>[2x]MAGQLLFANFNQDNTSLAVGSKSGYKFFSLSSVDKLEQIYECTDTEDVCIVERLFSSSLVAIVSLKAPRKLKVCHFKKGTEICNYSYSNTILAVKLNRQRLIVCLEESLYIHNIRDMKVLHTIRETPPNPAGLCALSINNDNCYLAYPGSATIGEVQVFDTINLRAANMIPAHDSPLAALAFDASGTKLATASEKGTVIRVFSIPEGQKLFEFRRGVKRCVSICSLAFSMDGMFLSASSNTETVHIFKLETVGSGSFNQGRAFATVRLPFCGHKNICSLATIQKIPRLLVGAADGYLYMYNLDPQEGGECALMKQHRLDGSLET;>[2x]YAENEKDSRRRQARLQKELAEAAKE

The ATG12–5–16L1 complex is responsible for conjugating members of the ubiquitin-like ATG8 protein family to phosphatidylethanolamine in the growing autophagosomal membrane, known as the phagophore. ATG12–5–16L1 is recruited to the phagophore by a subset of the phosphatidylinositol 3-phosphate-binding seven-bladedß -propeller WIPI proteins. The two critical steps in autophagy initiation, PI 3-phosphorylation and LC3 lipidation, are connected to one another via a direct interaction between a subset of the PI(3)P-binding WIPI proteins and ATG16L1. PROPPINs bind to PI(3)P and PI(3,5)P2 headgroups through a conserved FRRG motif and bind tightly, but reversibly, to membranes using a hydrophobic loop in blade six that inserts into the membrane.

Here, we report the crystal structure of WIPI2d:ATG16L1 (207–230) complex at a 1.85 Å resolution. In order to generate a crystallizable form of WIPI2d, the flexible hydrophobic loop in blade six and the putatively disordered C-terminal region were deleted. The asymmetric unit contains two copies of the WIPI2d:ATG16L1 W2IR complex. As expected on the basis of the Hsv2 and WIPI3 structures, WIPI2d folds into a seven blade ß -propeller, with each blade containing four anti-parallel ß-strands. The ATG16L1 W2IR nestles between blades 2 and 3 of WIPI2d, burying ~550 Å2 of solvent-accessible surface area. The WIPI2d binding site for the ATG16L1 W2IR consists of a single deep groove with a mixed electropositive and hydrophobic character. Hydrophobic side chains of Leu 64, Phe 65, Leu 69, Val 83, Ile 92, Cys 93, Ile 124, and Met 127 on WIPI2d contribute to the hydrophobic surface of the groove. The surfaces of Leu 220 and Leu 224 of the ATG16L1 W2IR are buried in this interface. The side chains of WIPI2d His 85, Lys 88, Arg 108, and Lys 128 contribute to the electropositive character of the groove. The acidic side chains of Glu 226 and Glu 230 of ATG16L1 interact with the electropositive patch on WIPI2.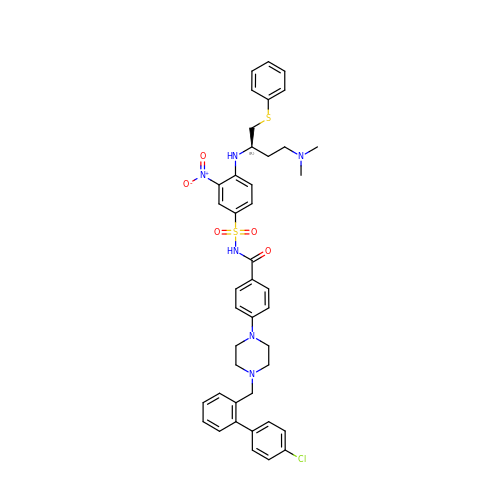4-{4-[(4'-CHLOROBIPHENYL-2-YL)METHYL]PIPERAZIN-1-YL}-N-{[4-({(1R)-3-(DIMETHYLAMINO)-1-[(PHENYLTHIO)METHYL]PROPYL}AMINO)-3-NITROPHENYL]SULFONYL}BENZAMIDE | C42 H45 Cl N6 O5 S2 | HPLNQCPCUACXLM-PGUFJCEWSA-N> AMPFEIEVLLPGELSPAETSALQKCEGKIITFSTLRHRASLVDIALSSYYINGAPPDTLSLLEAYRMRFAAVITRVIPGKLLAHAIGVGTPTPGLFIQNTSPVDLCNGDYICLLPPVFGSADSIRLDSVGLEIVFPLTIPQTL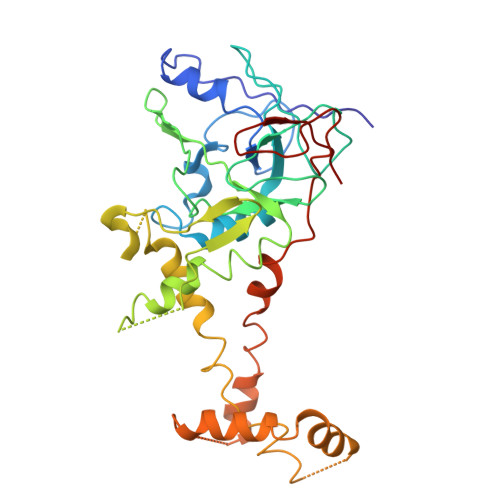MREIIAKVVARAVEDLNPDPDLNVLYYNGARLSLVADVQQLASDAAIRTLVLNLMFSINEGCLLILALIPRLLALGYVNALLQMQSVTREAAQLIHPEAPMLMRRLPIYETISSWISTSSRLGDTLGTRAILRVCVFDGPSTVHPGDRTAVIQV>MASGSCQGCEEDEETLKKLIVRLNNVQEGKQIETLVQILEDLLVFTYSEHASKLFQGKNIHVPLLIVLDSYMRVASVQQVGWSLLCKLIEVCPGTMQSLMGPQDVGNDWEVLGVHQLILKMLTVHNASVNLSVIGLKTLDLLLTSGKITLLILDEESDIFMLIFDAMHSFPANDEVQKLGCKALHVLFERVSEEQLTEFVENKDYMILLSALTNFKDEEEIVLHVLHCLHSLAIPCNNVEVLMSGNVRCYNIVVEAMKAFPMSERIQEVSCCLLHRLTLGNFFNILVLNEVHEFVVKAVQQYPENAALQISALSCLALLTETIFLNQDLEEKNENQENDDEGEEDKLFWLEACYKALTWHRKNKHVQEAACWALNNLLMYQNSLHEKIGDEDGHFPAHREVMLSMLMHSSSKEVFQASANALSTLLEQNVNFRKILLSKGIHLNVLELMQKHIHSPEVAESGCKMLNHLFEGSNTSLDIMAAVVPKILTVMKRHETSLPVQLEALRAILHFIVPGMPEESREDTEFHHKLNMVKKQCFKNDIHKLVLAALNRFIGNPGIQKCGLKVISSIVHFPDALEMLSLEGAMDSVLHTLQMYPDDQEIQCLGLSLIGYLITKKNVFIGTGHLLAKILVSSLYRFKDVAEIQTKGFQTILAILKLSASFSKLLVHHSFDLVIFHQMSSNIMEQKDQQFLNLCCKCFAKVAMDDYLKNVMLERACDQNNSIMVECLLLLGADANQAKEGSSLICQVCEKESSPKLVELLLNSGSREQDVRKALTISIGKGDSQIISLLLRRLALDVANNSICLGGFCIGKVEPSWLGPLFPDKTSNLRKQTNIASTLARMVIRYQMKSAVEEGTASGSDGNFSEDVLSKFDEWTFIPDSSMDSVFAQSDDLDSEGSEGSFLVKKKSNSISVGEFYRDAVLQRCSPNLQRHSNSLGPIFDHEDLLKRKRKILSSDDSLRSSKLQSHMRHSDSISSLASEREYITSLDLSANELRDIDALSQKCCISVHLEHLEKLELHQNALTSFPQQLCETLKSLTHLDLHSNKFTSFPSYLLKMSCIANLDVSRNDIGPSVVLDPTVKCPTLKQFNLSYNQLSFVPENLTDVVEKLEQLILEGNKISGICSPLRLKELKILNLSKNHISSLSENFLEACPKVESFSARMNFLAAMPFLPPSMTILKLSQNKFSCIPEAILNLPHLRSLDMSSNDIQYLPGPAHWKSLNLRELLFSHNQISILDLSEKAYLWSRVEKLHLSHNKLKEIPPEIGCLENLTSLDVSYNLELRSFPNEMGKLSKIWDLPLDELHLNFDFKHIGCKAKDIIRFLQQRLKKAVPYNRMKLMIVGNTGSGKTTLLQQLMKTKKSDLGMQSATVGIDVKDWPIQIRDKRKRDLVLNVWDFAGREEFYSTHPHFMTQRALYLAVYDLSKGQAEVDAMKPWLFNIKARASSSPVILVGTHLDVSDEKQRKACMSKITKELLNKRGFPAIRDYHFVNATEESDALAKLRKTIINESLNFKIRDQLVVGQLIPDCYVELEKIILSERKNVPIEFPVIDRKRLLQLVRENQLQLDENELPHAVHFLNESGVLLHFQDPALQLSDLYFVEPKWLCKIMAQILTVKVEGCPKHPKGIISRRDVEKFLSKKRKFPKNYMTQYFKLLEKFQIALPIGEEYLLVPSSLSDHRPVIELPHCENSEIIIRLYEMPYFPMGFWSRLINRLLEISPYMLSGRERALRPNRMYWRQGIYLNWSPEAYCLVGSEVLDNHPESFLKITVPSCRKGCILLGQVVDHIDSLMEEWFPGLLEIDICGEGETLLKKWALYSFNDGEEHQKILLDDLMKKAEEGDLLVNPDQPRLTIPISQIAPDLILADLPRNIMLNNDELEFEQAPEFLLGDGSFGSVYRAAYEGEEVAVKIFNKHTSLRLLRQELVVLCHLHHPSLISLLAAGIRPRMLVMELASKGSLDRLLQQDKASLTRTLQHRIALHVADGLRYLHSAMIIYRDLKPHNVLLFTLYPNAAIIAKIADYGIAQYCCRMGIKTSEGTPGFRAPEVARGNVIYNQQADVYSFGLLLYDILTTGGRIVEGLKFPNEFDELEIQGKLPDPVKEYGCAPWPMVEKLIKQCLKENPQERPTSAQVFDILNSAELVCLTRRILLPKNVIVECMVATHHNSRNASIWLGCGHTDRGQLSFLDLNTEGYTSEEVADSRILCLALVHLPVEKESWIVSGTQSGTLLVINTEDGKKRHTLEKMTDSVTCLYCNSFSKQSKQKNFLLVGTADGKLAIFEDKTVKLKGAAPLKILNIGNVSTPLMCLSESTNSTERNVMWGGCGTKIFSFSNDFTIQKLIETRTSQLFSYAAFSDSNIITVVVDTALYIAKQNSPVVEVWDKKTEKLCGLIDCVHFLREVTVKENKESKHKMSYSGRVKTLCLQKNTALWIGTGGGHILLLDLSTRRLIRVIYNFCNSVRVMMTAQLGSLKNVMLVLGYNRKNTEGTQKQKEIQSCLTVWDINLPHEVQNLEKHIEVRKELAEKMRRTSVE[4x];>[2x]MGSRDHLFKVLVVGDAAVGKTSLVQRYSQDSFSKHYKSTVGVDFALKVLQWSDYEIVRLQLWDIAGLERFAAMTRLYYRDASACVIMFDVTNATTFSNSQRWKQDLDSKLTLPNGEPVPCLLLANKCDLSPWAVSRDQIDRFSKENGFTGWTETSVKENKNINEAMRVLIEKMMRNS

Mutations in the LRRK2 gene, which encodes the leucine-rich repeat kinase 2 (LRRK2) protein, are among the most frequent genetic causes of late-onset PD and account for ~5% of familial and ~1% of sporadic cases. Most LRRK2-related PD mutations, such as G2019S (Gly2019→Ser), have increased kinase activity. Previous studies have suggested an emerging “Rab29–LRRK2–Rabs” cascade for LRRK2 signaling, in which GTP-bound Rab29 (Rab29•GTP) facilitates LRRK2 membrane recruitment and activation, then activated LRRK2 phosphorylates Rab GTPases, including Rab29 itself.

With a ~205 Å by 260 Å by 150 Å dimension, the Rab29–LRRK2 tetramer is an assembly with a twofold rather than fourfold symmetry, featuring two types of LRRK2 protomers: LRRK2peri (peripheral) and LRRK2cent (central). In addition, LRRK2peri directly interacts with LRRK2cent from the other asymmetric unit, with regions near the LRRK2peri ARM–ANK boundary packing against the LRRK2cent WD40 domain and the LRRK2peri ARM domain associated with the LRRK2cent ROC domain. The two LRRK2cent protomers pack in a “head-to-tail” mode through WD40–KIN interfaces. The catalytic halves of LRRK2cent and LRRK2peri show substantial conformational differences. The KIN domain of LRRK2cent has structural features of an active kinase. Critically, the LRRK2cent KIN domain adopts a closed conformation, with the αC helix positioned toward the active site and the “DYG motif’ flipped in. Lys1906 and Glu1920 form a salt bridge, an interaction blocked by Tyr2018 in the inactive conformation. There is a well-defined cryo-EM density for ATP in the active site, and the distance between Asp2017 and ATP shortens to 3.8 Å (from 13.8 Å in the inactive state), permitting ATP hydrolysis in the presence of substrates. LRRK2 activation features a striking dimer-of-asymmetric dimer assembly containing two active core subunits encased by two inactive peripheral protomers. The formation of active tetramers is Rab29-dependent because such an assembly was not observed with Rab32 or without Rab29 under similar experimental conditions.> MAHHHHHHVGTGSNDDDDKSPDPTQDVREPPALKYGIVLDAGSSHTSMFVYKWPADKENDTGIVGQHSSCDVQGGGISSYANDPSKAGQSLVRCLEQALRDVPRDRHASTPLYLGATAGMRLLNLTSPEATARVLEAVTQTLTQYPFDFRGARILSGQDEGVFGWVTANYL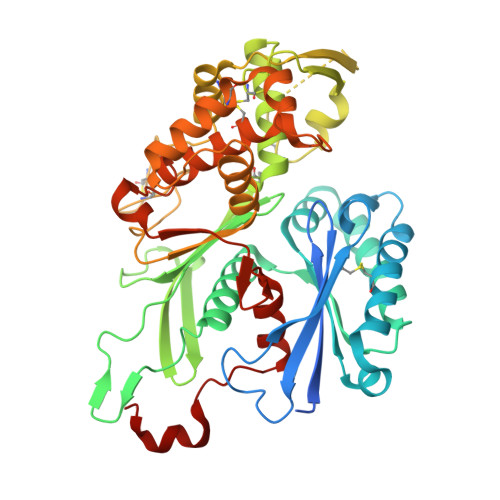LENFIKYGWVGRWIRPRKGTLGAMDLGGASTQITFETTSPSEDPGNEVHLRLYGQHYRVYTHSFLCYGRDQILLRLLASALQIHRFHPCWPKGYSTQVLLQEVYQSPCTMGQRPRAFNGSAIVSLSGTSNATLCRDLVSRLFNISSCPFSQCSFNGVFQPPVAGNFIAFSAFYYTVDFLTTVMGLPVGTLKQLEEATEITCNQTWTELQARVPGQKTRLADYCAVAMFIHQLLSRGYHFDERSFREVVFQKKAADTAVGWALGYMLNLTNLIPADLPGLRKGTHF>[2x]GCCCGGAUGAUCCUCAGUGGUCUGGGGUGCAGGCUUCAAACCUGUAGCUGUUUAGCGACAGAGUGGUUCAAUUCCACCUUUCGGGC

Specific tRNAs (tRNASec) are required for Sec biosynthesis and decoding, which are structurally distinct from canonical tRNAs. tRNASec is the only component of the Sec synthesis and insertion pathways that participates throughout all steps of Sec biosynthesis and decoding. For this multi-tasking, it has to interact with a number of different proteins, i.e. SerRS, PSTK, SelA/SecS and SelB/eEFSec. The unique interaction profile of tRNASec relies on special identity elements, which in part give rise to a number of distinct structural features but at the same time do not compromise the capacity of the molecule to act on the ribosome.

We have used a rational approach to engineer mouse tRNASec for crystallization and have determined its crystal structure at 2.0 Å resolution. Thus, as one strategy for crystallization of tRNASec, we deliberately deleted the single stranded 3′-GCCA overhang, generating ΔGCCAtRNASec with a blunt-ended acceptor stem. ΔGCCAtRNASec crystallized in space group P21 and yielded a diffraction data set to 2.0 Å resolution. There were two molecules of tRNASec in an asymmetric unit of the present crystal form (referred to as molecules A and B). Notably, the blunt-ended acceptor stem mediated crucial crystal packing contacts as intended. The first and last nucleotides of the variable arm (G45 and A48) form a water-mediated contact in one of the tRNASec molecules of the asymmetric unit of the present crystal structure (molecule A) and a direct non-canonical purine-purine pair in the other (molecule B). Comparison of the crystallographically independent mouse tRNASec structures and their comparison to the structures of human tRNASec alone or in complex with SecS showed that the variable and anticodon arms can adopt different relative orientation with respect to each other and with respect to the remainder of the molecule. In molecule A of the present structure, the anticodon stem consists of eight bps with a three-nt loop, comprising the three anticodon bases, U34, C35 and A36. In the anticodon loop of molecule B the reverse Watson-Crick bp between U33 and A37 is replaced by a partially opened reverse Hoogsteen pair, which comprises a single direct hydrogen bond between O2 of U33 and N6 of A37 and a water-mediated contact between N3 of U33 and N7 of A37. We therefore suggest that the conformation of the anticodon arm seen in molecule B reflects the functional conformation for UGA-decoding on the ribosome.ADENOSINE-2'-5'-DIPHOSPHATE 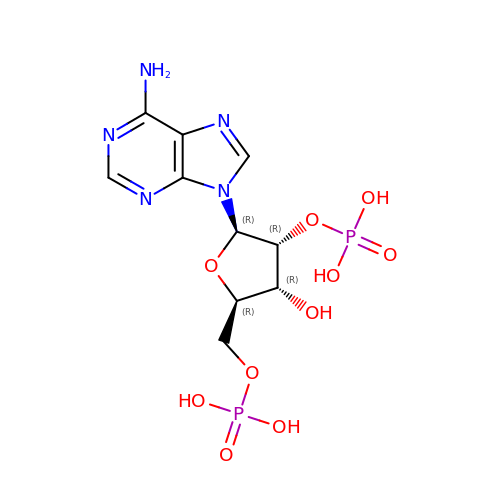| C10 H15 N5 O10 P2 | AEOBEOJCBAYXBA-KQYNXXCUSA-N>SPGIRMSVETIIERIKARVGAVDPNGPRKVLGVFQLNIKTASGVEQWIVDLKQLKVDQGVFASPDVTVTVGLEDMLAISGKTLTVGDALKQGKIELSGDADLA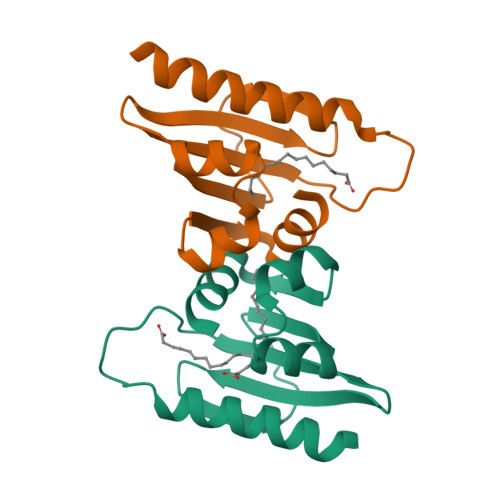AKLAEVI[2x]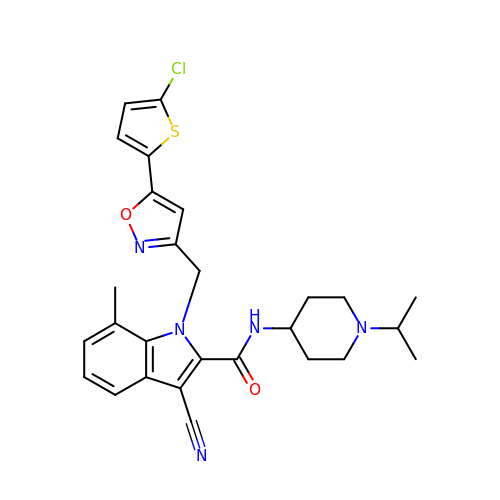1-{[5-(5-CHLORO-2-THIENYL)ISOXAZOL-3-YL]METHYL}-3-CYANO-N-(1-ISOPROPYLPIPERIDIN-4-YL)-7-METHYL-1H-INDOLE-2-CARBOXAMIDE | C27 H28 Cl N5 O2 S | MCLVKEPZVPUETD-UHFFFAOYSA-N>[2x]MKDDPKVHLEAKELWDQFHKRGTEMVITKSGRRMFPPFKVRCSGLDKKAKYILLMDIIAADDCRYKFHNSRWMVAGKADPEMPKRMYIHPDSPATGEQWMSKVVTFH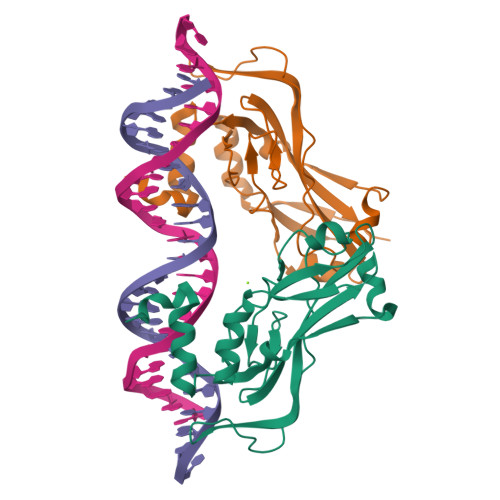KLKLTNNISDKHGFTILNSMHKYQPRFHIVRANDILKLPYSTFRTYLFPETEFIAVTAYQNDKITQLKIDNNPFAKGFRDTGNGRR> KNPKSDKFKVKRFHHIEFWCGDATNVARRFSWGLGMRFSAKSDLSTGNMVHASYLLTSGDLRFLFTAPYSPSLSAGEIKPTTTASIPSFDHGSCRSFFSSHGLGVRAVAIEVEDAESAFSISVANGAIPSSPPIVLNEAVTIAEVKLYGDVVLRYVSYKAEDTEKSEFLPGFERVEDASSFPLDYGIRRLDHAVGNVPELGPALTYVAGFTGFHQFAEFTADDVGTAESGLN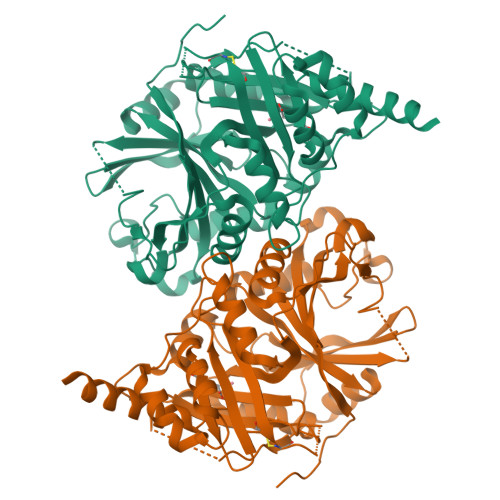WAVLASNDEMVLLPINEPVHGTKRKSQIQTYLEHNEGAGLQHLALMSEDIFRTLREMRKRSSIGGFDFMPSPPPTYYQNLKKRVGDVLSDDQIKECEELGILVDRDDQGTLLQIFTKPLGDRPTIFIEIIQRVGCMMKDEEGKAYQSGGCGGFGKGNFSELFKSIEEYEKTLE2,6-DIAMINO-HEXANOIC ACID AMIDE | C6 H16 N3 O 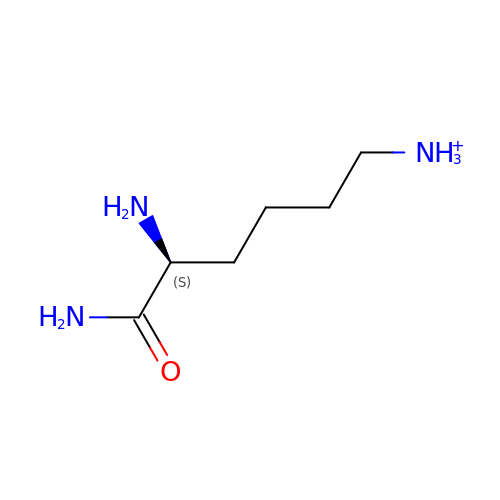| HKXLAGBDJVHRQG-YFKPBYRVSA-O>MSAEHVLTMLNEHEVKFVDLRFTDTKGKEQHVTIPAHQVNAEFFEEGKMFDGSSIGGWKGINESDMVLMPDASTAVIDPFFADSTLIIRCDILEPGTLQGYDRDPRSIAKRAEDYLRATGIADTVLFGPEPEFFLFDDIRFGASISGSHVAIDDIEGAWNSSTKYEGGNKGHRPGVKGGYFPVPPVDSAQDIRSEMCLVMEQMGLVVEAHHHEVATAGQNEVATRFNTMTKKADEIQIYKYVVHNVAHRFGKTATFMPKPMFGDNGSGMHCHMSLAK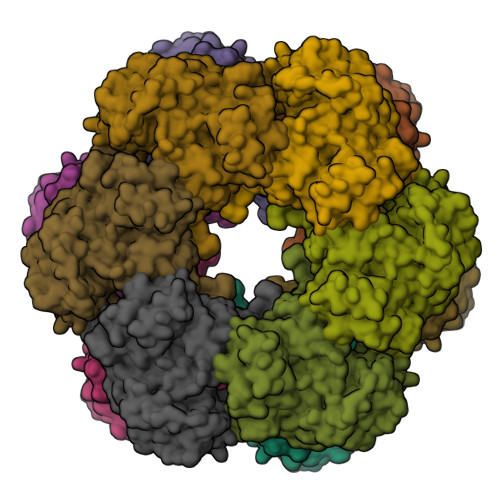NGTNLFSGDKYAGLSEQALYYIGGVIKHAKAINALANPTTNSYKRLVPGYEAPVMLAYSARNRSASIRIPVVASPKARRIEVRFPDPAANPYLCFAALLMAGLDGIKNKIHPGEPMDKNLYDLPPEEAKEIPQVAGSLEEALNALDLDREFLKAGGVFTDEAIDAYIALRREEDDRVRMTPHPVEFELYYSV[12x]In this system, thousands of copies of transmembrane (TM) chemoreceptors, the histidine autokinase CheA and adaptor protein CheW, form highly ordered structures known as chemosensory arrays, which cooperatively integrate the sensory inputs of multiple receptors to regulate the autophosphorylation activity of CheA. Core signaling units (CSU) of the chemosensory array contain six receptor dimers, organized as two trimers of dimers (TODs), a single CheA dimer and two CheW adaptor proteins. MCP molecules contain a periplasmic ligand-binding domain (LBD), TM four-helix bundle, and cytoplasmic kinase control domain. CheA functions as a homodimer in the CSU; each protomer comprises five domains (P1–P5) joined by flexible linkers.

In this study, we present the structure of the complete CSU from phage φX174 E protein lysed Escherichia coli cells, determined using cryo-electron tomography and sub-tomogram averaging to 12-Å resolution. The map of the full CSU, determined at an overall resolution of 12 Å, clearly resolves six full-length chemoreceptor dimers (red), a central CheA dimer containing distinct regions for P3–P5 (blue), four CheW monomers (orange and yellow), and the lipid bilayer headgroups (gray). In the periplasmic-focused map, the ellipsoidal shape of the individual LBDs became prominent and clearly indicated the orientation of each LBD, a feature not discernible in previous studies. Using AlphaFold2, we further predict the atomic structures of the CSU’s constituent proteins as well as key protein-protein interfaces, enabling the assembly an all-atom CSU model, which we conformationally refine using our cryo-electron tomography map. The constituent models were assembled via rigid docking using the predicted interfaces and our cryoET map to produce a preliminary model of the CSU, which was subsequently refined using molecular dynamics flexible fitting (MDFF). The resulting trajectory identified interactions between two co-planar clusters of charged residues on the Tsr LBDs, involving K99, E102, and K103 on helix 2 (cluster 1) as well as E124, K126, R127, and D130 on helix 3 (cluster 2). Rather, these interactions appear to form a pseudo-lattice by which the Tsr LBDs roughly maintain their relative orientations and inter-domain distances. The P5 regulatory domains are rotated slightly compared to the orientation required to form interface I with CheW. Intriguingly, the P1 domains were observed to form a dimer wedged between the two P4 domains where the aforementioned excess density in our cryoET map is localized. The P1 domains themselves are predicted to interact in an anti-parallel fashion mediated by P1 helices A and B, such that the substrate histidines face away from the P4 catalytic site and toward the P1/P1′ interface. The interaction between P1 and P4 is primarily mediated by a string of oppositely charged residues residing on helix D and the C-terminus of helix A in P1 and the α3 helix in P4.

>RSNESTSIRVAVEKVDQLINLVGELVITQSMLAQRSSELDPVNHGDLITSMGQLQRNARDLQESVMSIRMMPMEYVFSRYPRLVRDLAGKLGKQVELTLVGSSTELDKSLIERIIDPLTHLVRNSLDHGIELPEKRLAAGKNSVGNLILSAEHQGGNICIEVTDDGAGLNRERILAKAASQGLTVSENMSDDEVAMLIFAPGFSTAEQVTDVSGRGVGMDVVKRNIQKMGGHVEIQSKQGTGTTIRILLPLTLAILDGMSVRVADEVFILPLNAVMESLQPREADLHPLAGGERVLEVRGEYLPIVELWKVFNVAGAKTEATQGIVVILQSGGRRYALLVDQLIGQHQVVVKNLESNYRKVPGISAATILGDGSVALIVDVSALQAINREQ[2x];>[2x]MSMDISDFYQTFFDEADELLADMEQHLLVLQPEAPDAEQLNAIFRAAHSIKGGAGTFGFSVLQETTHLMENLLDEARRGEMQLNTDIINLFLETKDIMQEQLDAYKQSQEPDAASFDYICQALRQLALEAK;>SGQEFLVFTLGDEEYGIDILKVQEIRGYDQVTRIANTPAFIKGVTNLRGVIVPIVDLRIKFSQVDVDYNDNTVVIVLNLGQRVVGIVVDGVSDVLSLTAEQIRPAPEFAVTLSTEYLTGLGALGDRMLILVNIEKLLNSEEMA[4x];>MLKRIKIVTSLLLVLAVFGLLQLTSGGLFFNALKNDKENFTVLQTIRQQQSTLNGSWVALLQTRNTLNRAGIRYMMDQNNIGSGSTVAELMESASISLKQAEKNWADYEALPRDPRQSTAAAAEIKRNYDIYHNALAELIQLLGAGKINEFFDQPTQGYQDGFEKQYVAYMEQNDRLHDIAVSDNNASYSQAMWILVGVMIVVLAVIFAVWFGIKASLVAPMNRLIDSIRHIAGGDLVKPIEVDGSNEMGQLAESLRHMQGELMRTVGDVRNGANAIYSGASEIATGNNDLSSRTEQQAASLEETAASMEQLTATVKQNAENARQASHLALSASETAQRGGKVVDNVVQTMRDISTSSQKIADIISVIDGIAFQTNILALNAAVEAARAGEQGRGFAVVAGEVRNLAQRSAQAAREIKSLIEDSVGKVDVGSTLVESAGETMAEIVSAVTRVTDIMGEIASASDEQSRGIDQVGLAVAEMDRVTQQNAALVEESAAAAAALEEQASRLTEAVAVFR[12x]> MGHHHHHHQQLASFLSGTWQSGRGRSRLIHHAISGEALWEVTSEGLDMAAARQFAIEKGAPALRAMTFIERAAMLKAVAKHLLSEKERFYALSAQTGATRADSWVDIEGGIGTLFTYASLGSRELPDDTLWPEDELIPLSKEGGFAARHLLTSKSGVAVHINAFNFPCWGMLEKLAPTWLGGMPAIIKPATATAQLTQAMVKSIVDSGLVPEGAISLICGSAGDLLDHLDSQDVVTFTGSAATGQMLRVQPNIVAKSIPFTMEADSLNCCVLGEDVTPDQPEFALFIREVVREMTTKAGQKCTAIRRIIVPQALVNAVSDALVARLQKVVVGDPAQEGVKMGALVNAEQRADVQEKVNILLAAGCEIRLGGQADLSAAGAFFPPTLLYCPQPDETPAVHATEAFGPVATLMPAQNQRHALQLACAGGGSLAGTLVTADPQIAR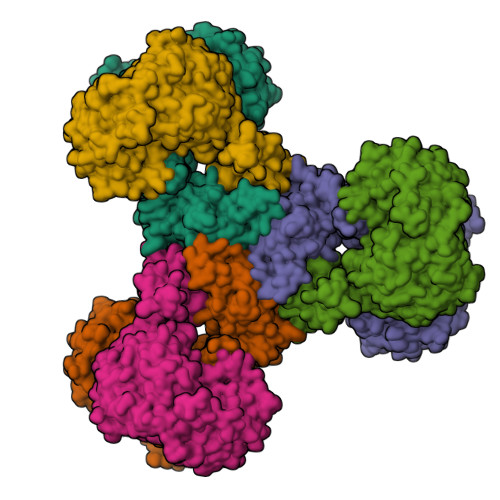QFIADAARTHGRIQILNEESAKESTGHGSPLPQLVHGGPGRAGGGEELGGLRAVKHYMQRTAVQGSPTMLAAISKQWVRGAKVEEDRIHPFRKYFEELQPGDSLLTPRRTMTEADIVNFACLSGDHFYAHMDKIAAAESIFGERVVHGYFVLSAAAGLFVDAGVGPVIANYGLESLRFIEPVKPGDTIQVRLTCKRKTLKKQRSAEEKPTGVVEWAVEVFNQHQTPVALYSILTLVARQHGDFVD> MARQNSAAKTTAKSKTDPATEKPKDD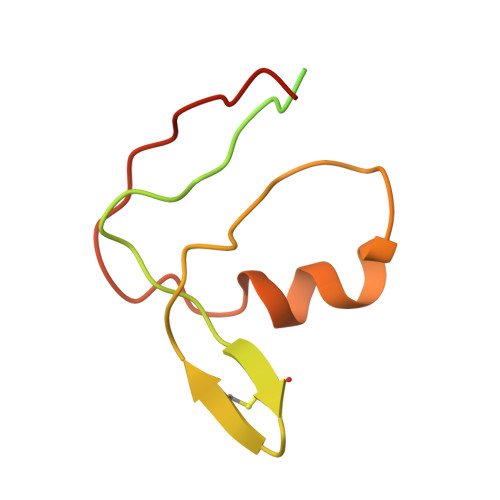TLPDSTDDASPTAPETPATKPDSASDEVEGVFVRATVERRCRAGFCFDKEGQGFADGVLSDEQLEALESDPLLKVERCTFSGNQEGE>[2x]MQKAVVMDEQAIRRALTRIAHEIIERNKGIDGCVLVGIKTRGIYLARRLAERIEQIEGASVPVGELDITLYRDDLTVKTDDHEPLVKGTNVPFPVTERNVILVDDV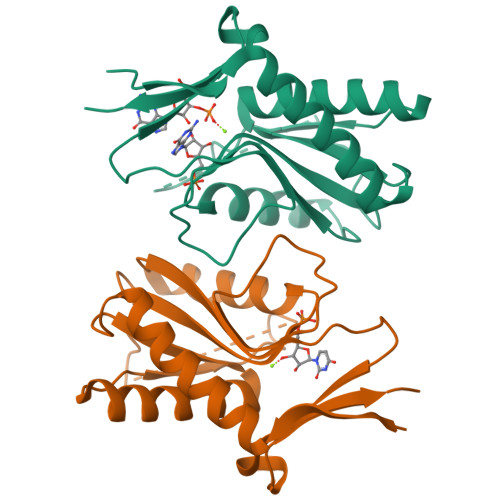LFTGRTVRAAMDAVMDLGRPARIQLAVLVDRGHRELPIRADFVGKNVPTSRSELIVVELSEVDGIDQVSIHEK>[4x]MAVKVIVTDMDGTFLNDAKTYNQPRFMAQYQELKKRGIKFVVASGNQYYQLISFFPELKDEISFVAENGALVYEH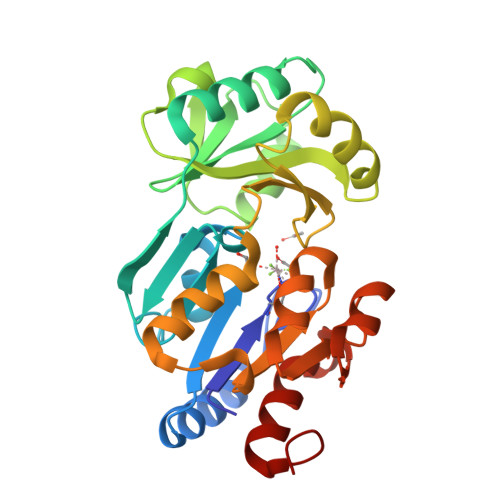GKQLFHGELTRHESRIVIGELLKDKQLNFVACGLQSAYVSENAPEAFVALMAKHYHRLKPVKDYQEIDDVLFKFSLNLPDEQIPLVIDKLHVALDGIMKPVTSGFGFIDLIIPGLHKANGISRLLKRWDLSPQNVVAIGDSGNDAEMLKMARYSFAMGNAAENIKQIARYATDDNNHEGALNVIQAVLDNTYPFNS> MRVNNGLTPQELEAYGISDVHDIVYNPSYDLLYQEELDPSLTGYERGVLTNLGAVAVDTGIFTGRSPKDKYIVRDDTTRDTFWWADKGKGKNDNKPLSPETWQHLKGLVTRQLSGKRLFVVDAFCGANPDTRLSVRFITEVAWQAHF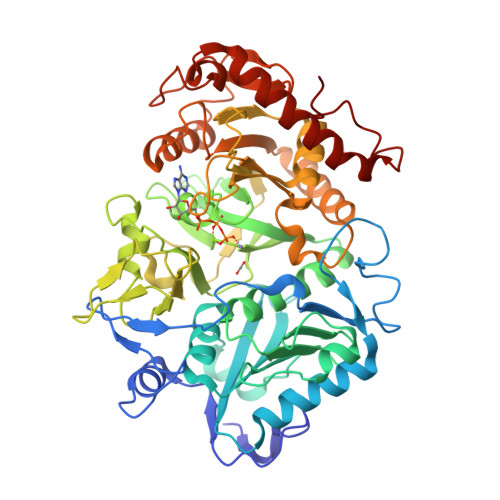VKNMFIRPSDEELAGFKPDFIVMNGAKCTNPQWKEQGLNSENFVAFNLTERMQLIGGTWYGGEMKKGMFSMMNYLLPLKGIASMHCSANVGEKGDVAVFFGLSGTGKTTLSTDPKRRLIGDDEHGWDDDGVFNFEGGCYAKTIKLSKEAEPEIYNAIRRDALLENVTVREDGTIDFDDGSKTENTRVSYPIYHIDNIVKPVSKAGHATKVIFLTADAFGVLPPVSRLTADQTQYHFLSGFTAKLAGTERGITEPTPTFSACFGAAFLSLHPTQYAEVLVKRMQAAGAQAYLVNTGWNGTGKRISIKDTRAIIDAILNGSLDNAETFTLPMFNLAIPTELPGVDTKILDPRNTYASPEQWQEKAETLAKLFIDNFDKYTDTPAGAALVAAGPKL> VFLCPGLLKGVYQSEHLFESDHQSGAWCKDPLQASDKIYY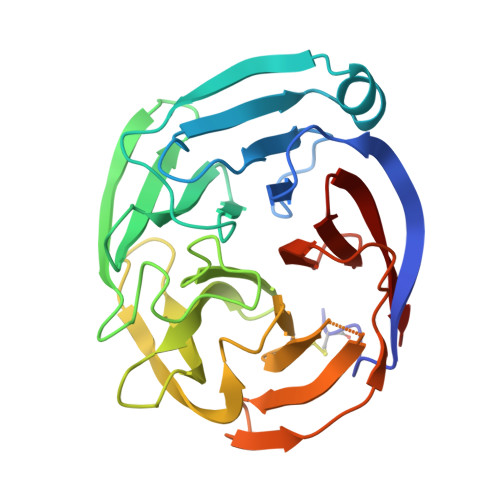MPWTPYRTDTLTEYSSKDDFIAGRPTTTYKLPHRVDGTGFVVYDGALFFNKERTRNIVKFDLRTRIKSGEAIIANANYHDTSPYRWGGKSDIDLAVDENGLWVIYATEQNNGKIVISQLNPYTLRIEGTWDTAYDKRSASNAFMICGILYVVKSVYEDDDNEATGNKIDYIYNTDQSKDSLVDVPFPNSYQYIAAVDYNPRDNLLYVWNNYHVVKYSLDFG>[4x]MGHHHHHHHHHHSSGHIDDDDKHTSLEVLFQGPHMPASQDKLDVPPGPYHFSEQVGHLLRRAYQRHVAIFQQTIPDSKLTAAQFVVLCALRDQGACSLVDVVKATAIDQATVRGVIERLKARKLLAVSHDPADRRKVLVTLTPDGRALVEEMVPFAEQITQSTFGGLNPAERVAIVYLLRKMSDADDLVGRQSDS

BpsR is a member of the MarR family of bacterial transcriptional regulators. MarR proteins often repress genes involved in the response to organic compounds, environmental stresses, and virulence factors. They are obligate homodimers and many are responsive to ligand binding. Recently, we and others have shown that BpsR controls the growth of B. bronchiseptica by repressing genes involved in nicotinic acid (NA) degradation. BpsR repression is relieved by binding of 6-hydroxynicotinic acid (6HNA), allowing tight regulation of the pathway to control NA metabolism according to the needs and environment of the bacterium.

BpsR crystallized the in the primitive orthorhombic space group (P212121) with 2 dimers in the asymmetric unit. The secondary structure of the protein is primarily α-helical composed of 6 α-helices and 2 β-strands per monomer. BpsR contains a winged Helix-turn-Helix (wHtH) domain for DNA binding. In the dimer, the two wHtH motifs are positioned in tandem to one another to create a DNA binding surface. The overall structure of the dimer is similar to other members of the MarR family of transcriptional regulators. The RMSD between BpsR and ecMarR is 1.38 Å (over 129 Cα atoms) which is indicative of high structural similarity. The model suggests that helix α4, from the HTH domain, inserts into DNA major groove and likely functions in DNA sequence recognition. The β hairpin wing motif extents away from the protein, along the DNA helix, to provide interactions with the phosphodiester backbone and the minor groove. Although the DNA sequence for BpsR binding is likely different, residues Thr76, Arg79, Gln83, Arg84, Lys86 within helix α4 extend towards the DNA bases within the major groove, providing potential sequence specific interactions. Within the wing region, Arg100, Arg101, and Lys102 interact with the DNA phosphate groups in the minor groove also contributing to the stability of the recognition helix interactions within the major groove.>MKGQTQRSVLLCKVVGACGVGKSAFLQAFLGRGLGHQDTREQPPGYAIDTVQVNGQEKYLILCEVGTDGLLATSLDATCDVACLMFDGSDPKSFAHCASVYKHHYMDGQTPCLFVSSKADLPEGVAVSGPSPAEFCRKHRLPAPVPFSCAGPAEPSTTIFTQLATMAAFPHLVHAELHPSSLEHHHHHH[3x]

Human Miro1 and Miro2 (hMiro1, hMiro2, also called RhoT1 and RhoT2) are MOM protein homologs that play a critical role in mitochondrial trafficking38394041424344. Both associate with Parkin upon mitochondrial depolarization and are ubiquitinated on multiple lysines18374546. Here, we demonstrate that the cGTPase domain is necessary and sufficient for efficient ubiquitination of either hMiro1 or hMiro2 by p-S65 Parkin. We also find that despite considerable similarities between these two substrates, Parkin modifies hMiro1 much more robustly than hMiro2.

To better understand the difference in ubiquitination efficiency between hMiro1 and hMiro2, we first determined the crystal structures of the isolated cGTPase domains of both proteins to high resolution (hMiro1-C: 2.25 Å; hMiro2-C: 1.69 Å). The overall folds of the hMiro1 and hMiro2 cGTPase domains are quite similar (rmsd 0.78 Å over 129 Cα atoms). Unexpectedly, both domains crystallized as symmetric dimers. The dimer interface is a highly conserved hydrophobic surface along one face of the cGTPase domain, which, in the intact hMiro1-BC structure, forms the interface with the second hidden EF hand (hEF2). The residues of the cGTPase domain that interact with hEF2 are structurally conserved in the hMiro1 and hMiro2 homologs, and a structure-based alignment of the four residues of the hMiro1 hEF2 at the core of the hEF2/cGTPase interface shows they are 100% conserved in hMiro2 hEF2. Interestingly, although the same conserved residues mediate dimerization in hMiro1-C and hMiro2-C, their dimer relationships differ significantly. We performed size exclusion chromatography with in-line multi-angle light scattering (SEC-MALS) and confirmed that both hMiro1-C and hMiro2-C dimerize in solution. We next sought to establish a structural basis for the difference in ubiquitination between hMiro1 and hMiro2, and the preference p-S65 Parkin exhibits for targeting K572 in hMiro1. hMiro2 contains a glutamine, Q569, at the position equivalent to hMiro1’s K572. Beyond the location of this key target lysine, the electrostatic surface potentials of the cGTPase homologs are also markedly different, especially in the vicinity of K572/Q569. In contrast to the isolated hMiro1 cGTPase, however, the isolated cGTPase of hMiro2 (hMiro2-C) was only weakly modified, suggesting the cGTPase domain of hMiro2 may not itself contain efficiently modified lysines.tert-butyl {(3R)-3-[(1H-tetrazol-5-yl)carbamoyl]-1-[3-(trifluoromethyl)benzoyl]-2,3-dihydro-1H-indol-3-yl}carbamate 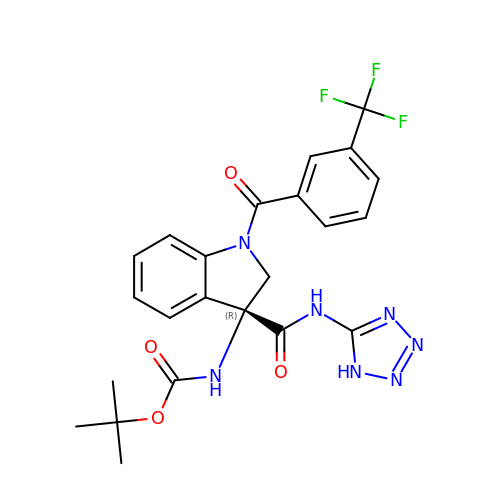| C23 H22 F3 N7 O4 | RFHIEPXMXRQDKW-QFIPXVFZSA-N>ANDAPIVLLHGFTGWGREEMFGFKYWGGVRGDIEQWLNDNGYRTYTLAVGPLSSNWDRACEAYAQLVGGTVDYGAAHAAKHGHARFGRTYPGLLPELKRGGRIHIIAHSQGGQTARMLVSLLENGSQEEREYAKAHNVSLSPLFEGGHHFVLSVTTIATPHDGTTLVNMVDFTDRFFDLQKAVLKAAAVASNVPYTSQVYDFKLDQWGLRRQPGESFDQYFERLKRSPVWTSTDTARYDLSVPGAEKLNQWVKASPNTYYLSFATERTYRGALTGNYYPELGMNAFSAVVCAPFLGSYRNA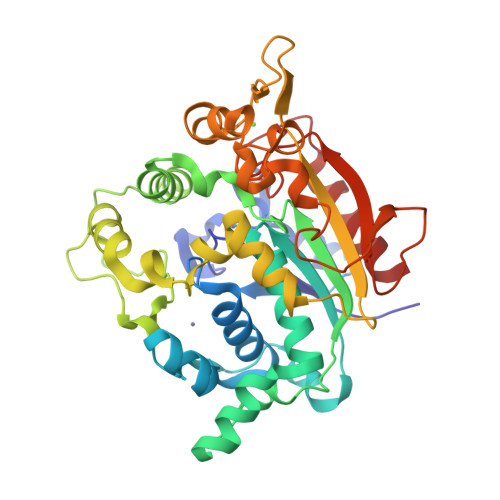TLGIDDRWLENDGIVNTFSMNGPKRGSTDRIVPYDGTIKKGVWNDMGTYNVDHLEVIGVDPNPLFDIRAFYLRLAEQLAS[2x]>MKTPTIPTLLGPDGMTSLREYAGYHGGGSGFGGQLRSWNPPSESVDAALLPNFTRGNARADDLVRNNGYAANAIQLHQDHIVGSFFRLSHRPSWRYLGIGEEEARAFSREVEAAWKEFAEDDCCCIDVERKRTFTMMIREGVAMHAFNGELFVQATWDTSSSRLFRTQFRMVSPKRISNPNNTGDSRNCRAGVQINDSGAALGYYVSEDGYPGWMPQKWTWIPRELPGGRASFIHVFEPVEDGQTRGANVFYSVMEQMKMLDTLQNTQLQSAIVKAMYAATIESELDTQSAMDFILGANSQEQRERLTGWIGEIAAYYAAAPVRLGGAKVPHLMPGDSLNLQTAQDTDNGYSVFEQSLLRYIAAGLGVSYEQLSRNYAQMSYSTARASANESWAYFMGRRKFVASRQASQMFLCWLEEAIVRRVVTLPSKARFSFQEARSAWGNCDWIGSGRMAIDGLKEVQEAVMLIEAGLSTYEKECAKRGDDYQEIFAQQVRETMERRAAGLKPPAWAAAAFESGLRQSTEEEKSDSRAA[12x];>[30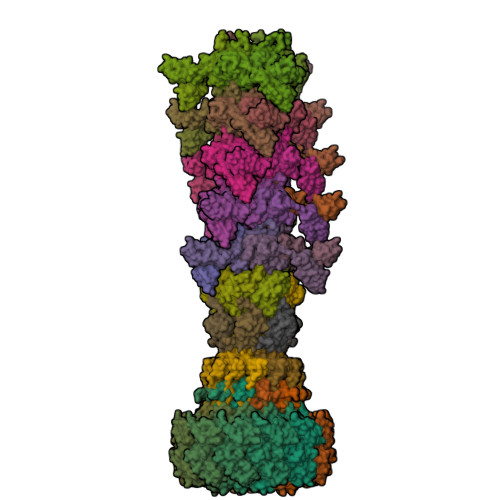x]MPVPNPTMPVKGAGTTLWVYKGSGDPYANPLSDVDWSRLAKVKDLTPGELTAESYDDSYLDDEDADWTATGQGQKSAGDTSFTLAWMPGEQGQQALLAWFNEGDTRAYKIRFPNGTVDVFRGWVSSIGKAVTAKEVITRTVKVTNVGRPSMAEDRSTVTAATGMTVTPASTSVVKGQSTTLTVAFQPEGVTDKSFRAVSADKTKATVSVSGMTITVNGVAAGKVNIPVVSGNGEFAAVAEITVTAS;>MKHTELRAAVLDALEKHDTGATFFDGRPAVFDEADFPAVAVYLTGAEYTGEELDSDTWQAELHIEVFLPAQVPDSELDAWMESRIYPVMSDIPALSDLITSMVASGYDYRRDDDAGLWSSADLTYVITYEM[6x];>MTRQEELAAARAALHDLMTGKRVATVQKDGRRVEFTATSVSDLKKYIAELEVQTGMTQRRRGPAGFYV[12x];>MADFDNLFDAAIARADETIRGYMGTSATITSGEQSGAVIRGVFDDPENISYAGQGVRVEGSSPSLFVRTDEVRQLRRGDTLTIGEENFWVDRVSPDDGGSCHLWLGRGVPPAVNRRR[6x]>MTNIAKAQPKLYVMDNGRMRMDKNWMIAMHNPATIANPNAPTEFIEFPIYTVLIDHPEGKILFDTSCNPDSMGAQGRWGEATQSMFPWTASEECYLHNRLEQLKVRPEDIKFVIASHLHLDHAGCLEMFTNATIIVHEDEFSGALQTYARNQTEGAYIWGDIDAWIKNNLNWRTIKRDEDNIVLAEGIKILNFGSGHAWGMLGLHVQLPEKGGIILASDAVYSAESYGPPIKPPGIIYDS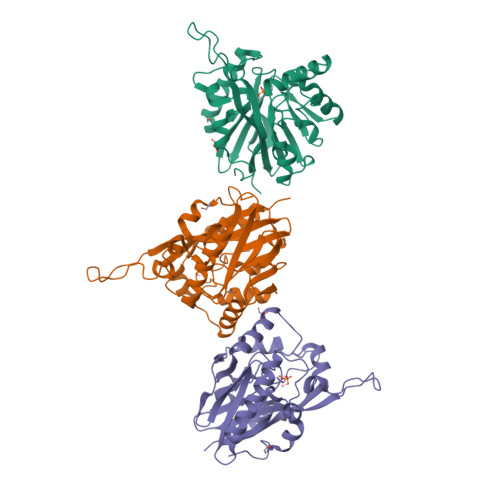LGFVRSVEKIKRIAKETNSEVWFGHDSEQFKRFRKSTEGYYE[3x]>MTKEKISVTVDAAVLAAIDADARAAGLNRSEMIEQALRNEHLRVALRDYTAKTVPA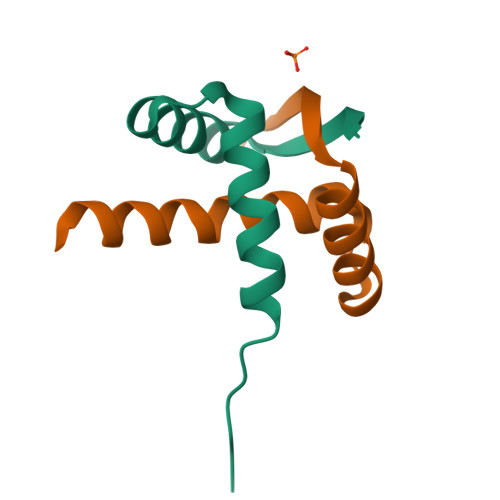LDIDAYAQRVYQANRAAGS[2x]>[2x]MGARKASAGASRAATAGVRISHPQRLIDPSIQASKLELAEFHARYADLLLRDLRERPVSLVRGPDGIGGELFFQKHAARLKIPGIVQLDPALDPGHPPLLQIRSAEALVGAVQMGSIEFHTWNASLANLERPDRFVLDLDPDPALPWKRMLEATQLSLTLLDELGLRAFLKTSGGKGMHLLVPLERRHGWDEVKDFAQAISQHLARLMPERFSAVSGPRNRVGKIFVDYLRNSRGASTVA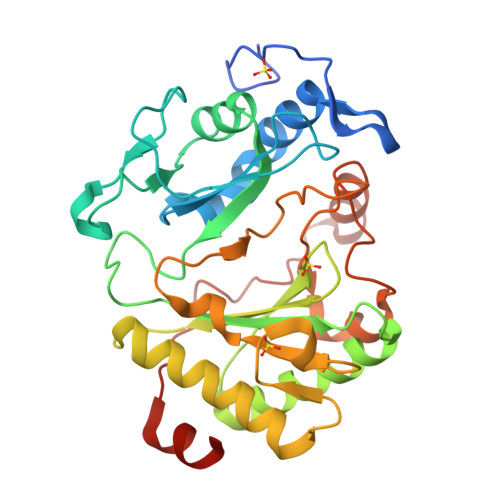AYSVRAREGLPVSVPVFREELDSLQGANQWNLRSLPQRLDELAGDDPWADYAGTRQRISAAMRRQLGRG> HMKQFEIVIEPIQTEQYREFTINEYQGAVVVFTGHVREWTKGV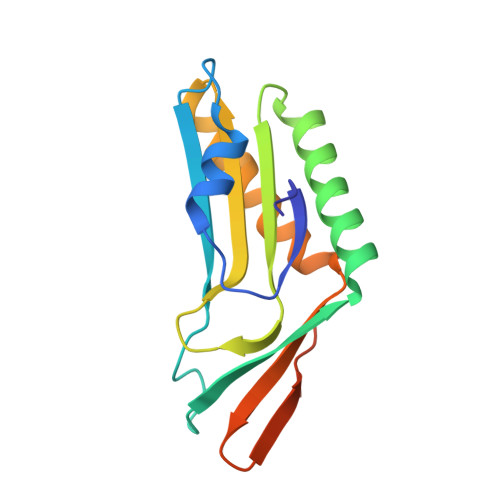KTEYLEYEAYIPMAEKKLAQIGDEINEKWPGTITSIVHRIGPLQISDIAVLIAVSSPHRKDAYRANEYAIERIKEIVPIWKKEIWEDGSKWQGHQKGNYEEAKREE> MGSSHHHHHSSGLVPRGSHMQMIAEIYYERGTIVVKGDAHVPHAKFDSRSGTYRALAFRYRDIIEYFESNGIEFVDNAADPIPTPYFDAEISLRDYQEKALERWLVDKRGCIVLPTGSGKTHVAMAAINELSTPTLIVVPTLALAEQWKERLGIFGEEYVGEFSGRIKELKPLTVSTYDSAYVNAEKL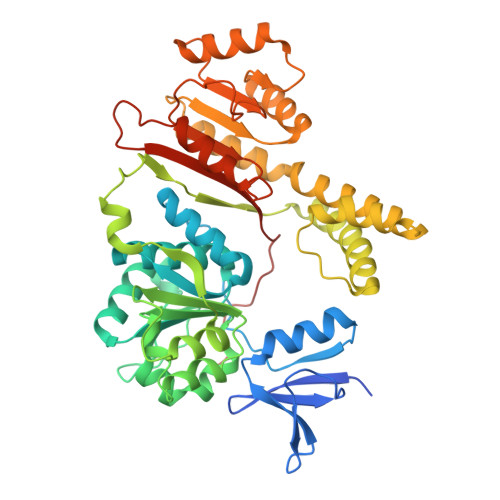GNRFMLLIFDEVHHLPAESYVQIAQMSIAPFRLGLTATFEREDGRHEILKEVVGGKVFELFPDSLAGKHLAKYTIKRIFVPLAEDERVEYEKREKVYKQFLRARGITLRRAEDFNKIVMASGYDERAYEALRAWEEARRIAFNSKNKIRKLREILERHRKDKIIIFTRHNELVYRISKVFLIPAITHRTSREEREEILEGFRTGRFRAIVSSQVLDEGIDVPDANVGVIMSGSGSAREYIQRLGRILRPSKGKKEAVLYELISRGTGEVNTARRRKNAAKGAA The TBC1D23 protein functions in membrane trafficking and is critical for human neuronal development. TBC1D23 is a recently characterized member of the TBC family and is conserved in many eukaryotic taxa. In mammalian cells, TBC1D23 is localized on the trans-Golgi network (TGN) and functions as an adaptor to capture the incoming endosome-derived vesicles. Unlike many members of the TBC family, TBC1D23 lacks the catalytic Arg-Gln residues and unlikely functions as an active GAP.

After screening many different expression constructs, we were able to obtain diffraction-quality crystals of the TBC1D23 N-terminal region (D23N) consisting of residues 1–460 and encompassing both the TBC and rhodanese domains. The crystal structure of D23N was determined by selenium single-wavelength anomalous diffraction (Se-SAD) and refined to a resolution of 2.5 Å. Each crystallographic asymmetric unit contains one D23N molecule, and the final model contains residues 14–298 (TBC domain, cyan) and residues 316–460 (rhodanese domain, yellow), connected by a short loop (amino acids [aa] 297–315; gold color), which adopts a 310-helix within its N-terminus. The TBC and rhodanese domains tightly pack against each other and bury a total solvent-accessible surface area of 1,350 Å2. The two domains together adopt a V-shaped structure, with the TBC domain forming the base and one arm and the rhodanese domain the other arm. Similar to other TBC-containing proteins, the TBC domain of TBC1D23 only compromises α-helices, which can be further divided into two subdomains: the amino-terminal domains containing α1–α7 and a carboxy-terminal subdomain spanning α8–α16. The rhodanese domain of TBC1D23 adopts α/β topology typical of a single rhodanese domain. In contrast with CDC25B, the putative active-site cysteine residue C399 is localized in the middle of β2 strand of the β-sheet, and its side chain is solvent-inaccessible. Thus, our structural analysis indicates that the rhodanese domain of TBC1D23 is unlikely to be an active phosphatase or sulfurtransferase. D23N possesses several deep pockets lining the center of its surface, with pocket 1 and 2 being predominately hydrophobic and pocket 3 consisting of both aromatic and negative charged residues.

> GWEKDLEEALEAGGCDLETLRNIIQGRPLPADLRAKVWKIALNVAGKGDSLASWDGILDLPEQNTIHKDCLQFIDQLSVPEEKAAELLLDIESVITFYCKSRNIKYSTSLSWIHLLKPLVHLQLPRSDLYNCFYAIMNKYIPRDCSQKGRPFHLFRLLIQYHEPELCSYLDTKKITPDSYALNWLGSLFACYCSTEVTQAIWDGYLQQADPFFIYFLMLIILVNAKEVILTQESDSKEEVIKFLENTPSSLNIEDIEDLFSLAQYYCSKTPASFRKDNHHLFGSTLLGIKDDDADLSQALCLAISVSEILQANQLQGEGVRFFVVDCRPAEQYNAGHLSTAFHLDSDLMLQNPSEFAQSVKSLLEAQKQSIESGSIAGGEHLCFMGSGREEEDMYMNMVLAHFLQKNKEYVSIASGGFMALQQHLADINVDGPENGYGHWIAST(2S)-1-{[(5-methylthiophen-2-yl)methyl]amino}propan-2-ol | C9 H15 N O S | 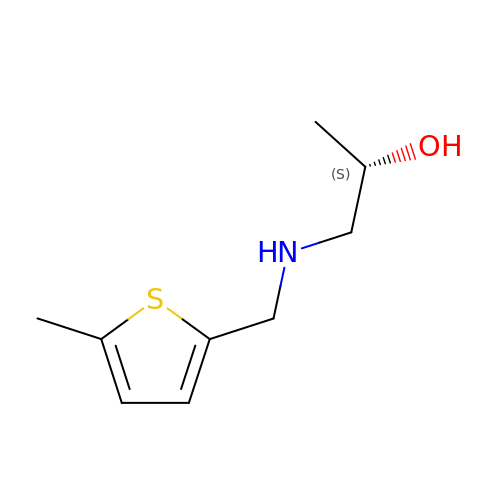JLVFMHMDKADIAM-ZETCQYMHSA-N In the case of the glutaredoxin that is the focus of this study, glutaredoxin A from the cyanobacterium Synechocystis sp. PCC 6803 serves as the preferred electron donor for the 2-electron reduction of arsenate to arsenite, catalyzed by arsenate reductase. As part of the thioredoxin superfamily, glutaredoxin A shares the characteristic thioredoxin fold. The structure of the wild-type protein is comprised of the major protein secondary structure elements: four α-helical segments, and four mixed parallel: anti-parallel β-strands that form a single β-pleated sheet. Our random mutagenesis approach has yielded four new crystal structures of glutaredoxin A, one for each of the following variants: R27L, A75I, A79S, and P84R.

The overall structure of the R27L variant is virtually indistinguishable from that of the wild-type protein. The RMSD (root-mean-square deviation) between both structures is 0.099 Å over all atoms, and the Leu27 substitution was confirmed in the refined experimental electron density. Arg27 occurs at the C-terminal end of α-helix 1 of the wild-type protein and potentially forms a H-bond with Tyr74. In addition, Arg27 occurs in a cluster of other basic residues (...K-R-K...), so it is likely that it is part of a localized positively charged patch on the surface of the protein. The leucine substitution would obviously disrupt this patch, but little else would be predicted to occur. Crystals of the wild-type protein diffract to 1.7 Å resolution, while the R27L mutation produced crystals that diffract X-rays to 1.2 Å resolution. The sizes of the crystals of the wild-type and R27L variants were similar, so the increase in diffraction cannot be explained by larger crystals. There is a possibility that more efficient hydrophobic packing between symmetry-related molecules, mediated by the leucine replacement, contributed to more efficient crystal packing. This observation is essentially what has been described as surface entropy reduction (SER). The R27L crystal structure lacks two neighbors; the A75I and A79S mutant have no net differences, while the P84R mutant adds three possible interactions.

> MRGSHHHHHHGSAVSAKIEIYTWSTCPFCMRALALLKLKGVEFQEYCIDGDNEAREAMAARANGKRSLPQIFIDDQHIGGCDDIYALDGAGKLDPLLHS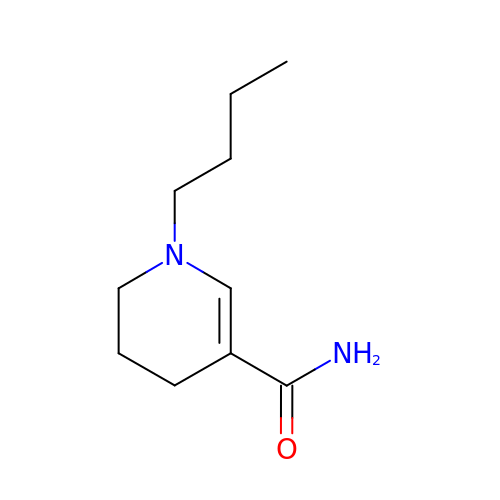1-butyl-1,4,5,6-tetrahydropyridine-3-carboxamide | C10 H18 N2 O | QWLZGRCLLUCDGU-UHFFFAOYSA-N>MATVAVVPAAGSGERLRAGRPKAFVTLGGTPLLEHALSGLRASGVIDRIVIAVPPALTDESKLVFGGEDSVIVSGGVDRTESVALALEAAGDAEFVLVHDAARALTPPALIARVVAALKEGHSAVVPGLAPADTIKAVDANGAVLGTPERAGLRAVQTPQGFHADVLRRAYARATAGGVTDDASLVEQLGTPVQIVDGDPLAFKIT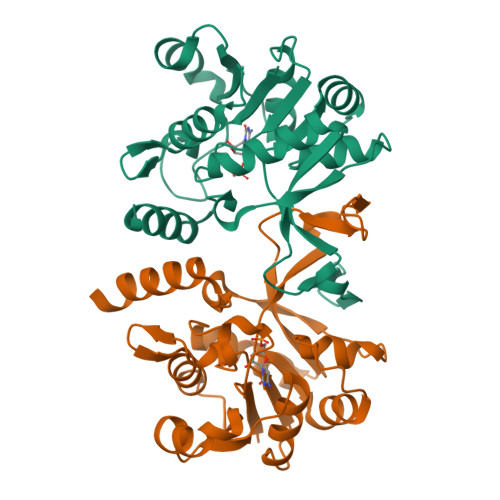TPLDLVLAEAVLAHHHH[2x]>[4x]SMKTKLMTLQDATGFFRDGMTIMVGGFMGIGTPSRLVEALLESGVRDLTLIANDTAFVDTGIGPLIVNGRVRKVIASHIGTNPETGRRMISGEMDVVLVPQGTLIEQIRCGGAGLGGFLTPTGVGTVVEEGK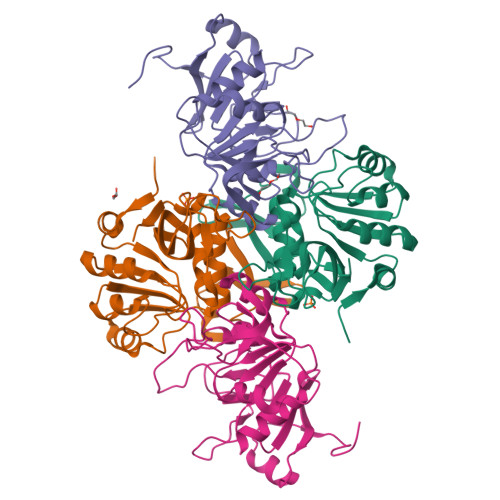QTLTLDGKTWLLERPLRADLALIRAHRCDTLGNLTYQLSARNFNPLIALAADITLVEPDELVETGELQPDHIVTPGAVIDHIIVSQESK;>[4x]MDAKQRIARRVAQELRDGDIVNLGIGLPTMVANYLPEGIHITLQSENGFLGLGPVTTAHPDLVNAGGQPCGVLPGAAMFDSAMSFALIRGGHIDACVLGGLQVDEEANLANWVVPGKMVPGMGGAMDLVTGSRKVIIAMEHCAKDGSAKILRRCTMPLTAQHAVHMLVTELAVFRFIDGKMWLTEIADGCDLATVRAKTEARFEVAADLNTQRGDLTHHHHHH> WNIHGKESCDVQLYIKRQSEHSILAGDPFELECPVKYCANRPHVTWCKLNGTTCVK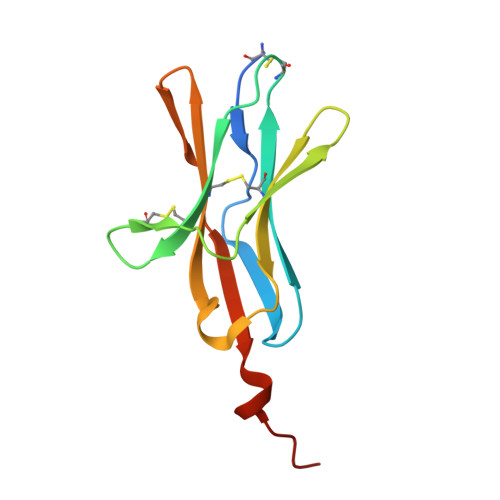LEDRQTSWKEEKNISFFILHFEPVLPNDNGSYRCSANFQSNLIESHSTTLYVTDVKHHHHHHHH> MDYTPHTEEEIREMLRRVGAASLEDLFAHLPKEILSPPIDLPEPLPEWKVLEELRRLAAQNLPAHKAFLGGGVRSHHVPPVVQALAARGEFLTAYTPYQPEVSQGVLQATFEYQTMIAELAGLEIANASMYDGATALAEGVLLALRET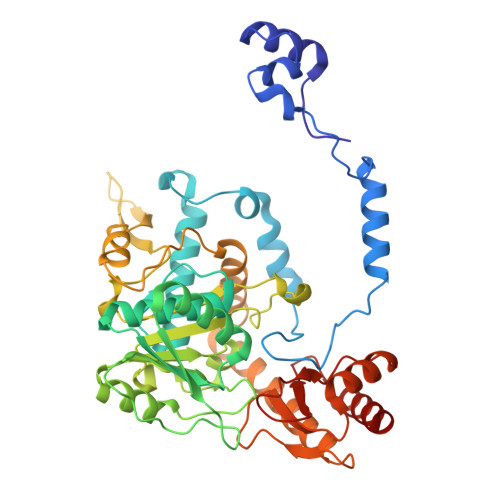GRMGVLVSQGVHPEYRAVLRAYLEAVGAKLLTLPLEGGRTPLPEVGEEVGAVVVQNPNFLGALEDLGPFAEAAHGAGALFVAVADPLSLGVLKPPGAYGADIAVGDGQSLGLPMGFGGPHFGFLATKKAFVRQLPGRLVSETVDVEGRRGFILTLQAREQYIRRAKAKSNITTNAQLTALMGAMYLAALGPEGLREVALKSVEMAHKLHALLLEVPGVRPFTPKPFFNEFALALPKDPEAVRRALAERGFHGATPVPREYGENLALFAATELHEEEDLLALREALKEVLA4-amino-N-{1-[(cyanomethyl)carbamoyl]cyclohexyl}-3-fluorobenzamide 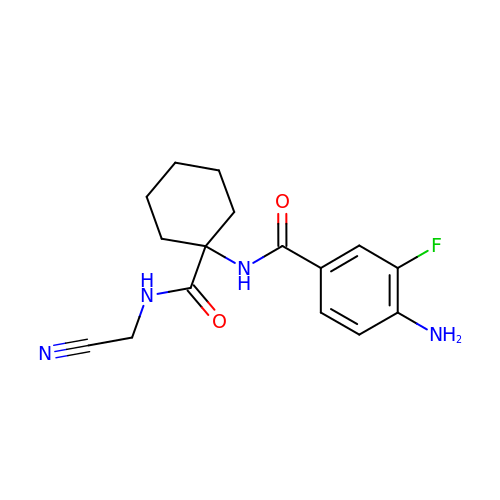| C16 H19 F N4 O2 | NEJGUCSKQVFSJQ-UHFFFAOYSA-N L-TREITOL | C4 H10 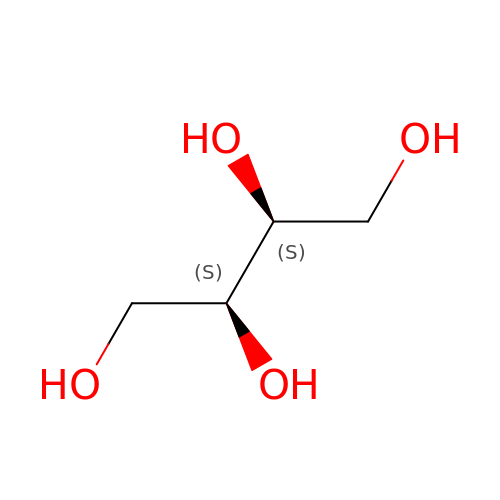O4 | UNXHWFMMPAWVPI-IMJSIDKUSA-N> GSHMSGIALSRLAQERKAWRKDHPFGFVAVPTKNPDGTMNLMNWECAIPGKK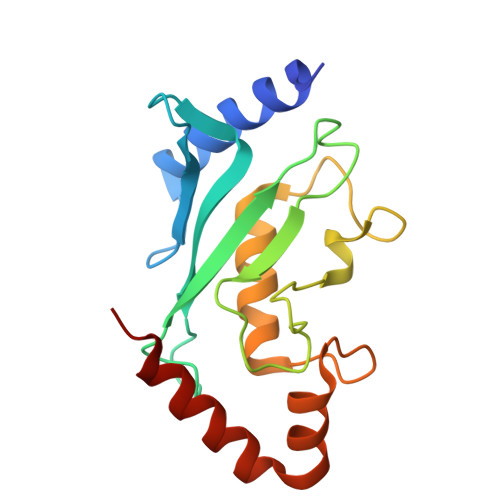GTPWEGGLFKLRMLFKDDYPSSPPKCKFEPPLFHPNVAPSGTVCLSILEEDKDWRPAITIKQILLGIQELLNEPNIQDPAQAEAYTIYCQNRVEYEKRVRAQAKKFAPS COA-S-TRIMETHYLENE-ACETYL-TRYPTAMINE | C36 H54 N9 O17 P3 S 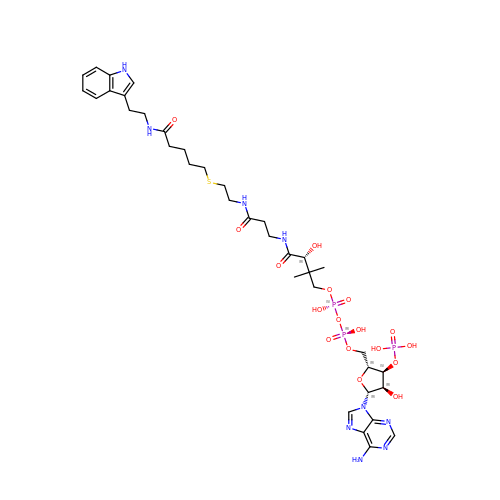| RFOXOYXMKJPZDH-VTINEICCSA-N> MRVLILGVNGFIGNHLTERLLREDHYEVYGLDIGSDAISRFLNHPHFHFVEGDISIHSEWIEYHVKKCDVVLPLVAIATPIEYTRNPLRVFELDFEENLRIIRYCVKYRKRIIFPSTSEVYGMCSDKYFDEDHSNLIVGPVNKPRWIYSVSKQLLDRVIWAYGEKEGLQFTLFRPFNWMGPRLDNLNAARIGSSRAITQLILNLVEGSPIKLIDGGKQKRCFTDIRDGIEALYRIIENAGNRCDGEIINIGNPENEASIEELGEMLLASFEKHPLRHHFPPFAGFRVVESSSYYGKGYQDVEH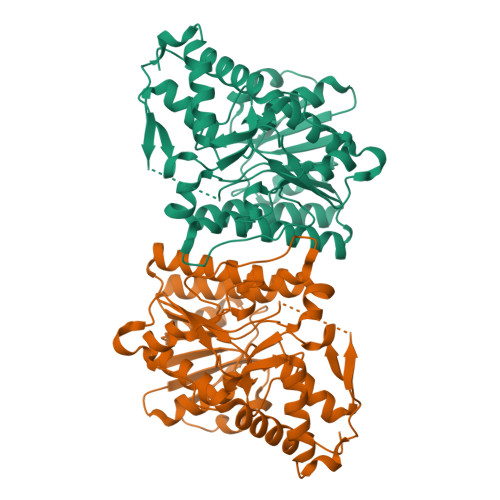RKPSIRNAHRCLDWEPKIDMQETIDETLDFFLRTVDLTDKPS> MSSHYEAPIRKPLVIGDKSYHDVTVDVAAPVEGPANKQWWIVFTIALVAFLWGLGCIIYTVSTGIGTWGLNKTVGWAWDITNFVWWVGIGHAGTLISAVLLLFRQRWRMAINRSAEAMTIFSVVQAGLFPIIHMGRPWLAYWVLPIPNQFGSLWVNFNSPLLWDVFAISTYLSVSLVFWWTGLLPDFAMLRDRAITPFNKRVYSILSFGWSGRAKDWQRFEEVSLVLAGLATPLVLSVHTIVSMDFATSVIPGWHTTIFPPYFVAGAVFSGFAMVNTLLIVMRKVSNLEAYITLQHIELMNIIIMITGSIVGVAYITELFVAWYSGVEYEQYAFLNRATGPYWWAYWSMMTCNVFSPQFMWFKKLRTSIMFSFIISIVVNIGMWFERFVIIVTSLHRDYLPSSWTMFSPTFVDIGIFIG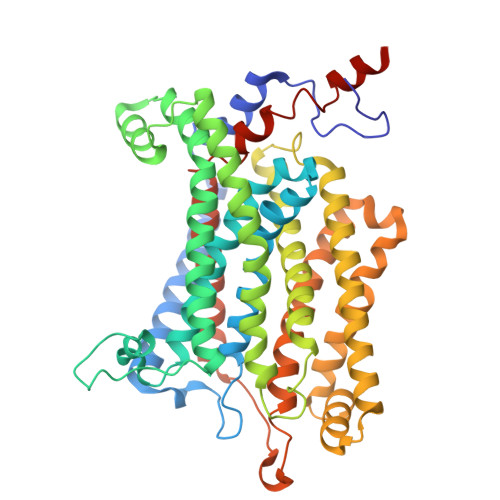TIGFFFVLFLLYSRTFPVIAQAEVKTILKGTGDNYIRERANKDSHHE> MALGTIGILSMFSVTCKSTDNNFWKSTFTSNNVNLFGDELSYNLIFVTLGIIDIWVGEMIKRVFVFCGEFRFINSRYDGRISFVVQQSF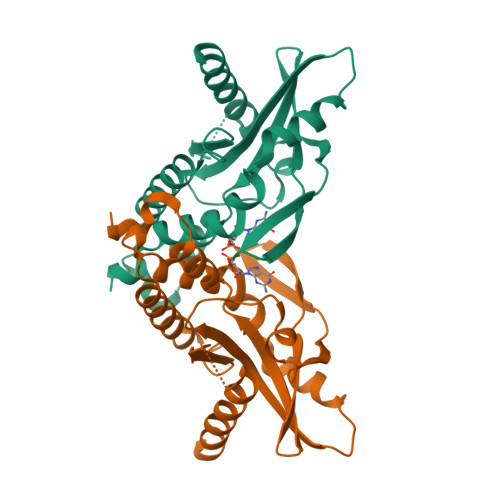CTKSNIPFLTLPILVAMLTYMNLHGDGMLLDPTKSEMSRVMEEQKLNVGHGLAWSYYFGYLRLIIPGLQSRMDSWKKGIDTARKSVVVPKLYLLIPKSCYCPPSITAADPQIKVAGVTPSFVANRAGNQRREYKNTVYCFEADKTDFYCLVEYATPILSLYEMSNSEEAGLSSFDRLRQMRTFVATLQEIINSNPETKDNCSLLVYDDKKFGDGEQSISMLIKDRIEKDLSDKALQMVDDFAKVVDGTNTDTISSKCANELTEDI>[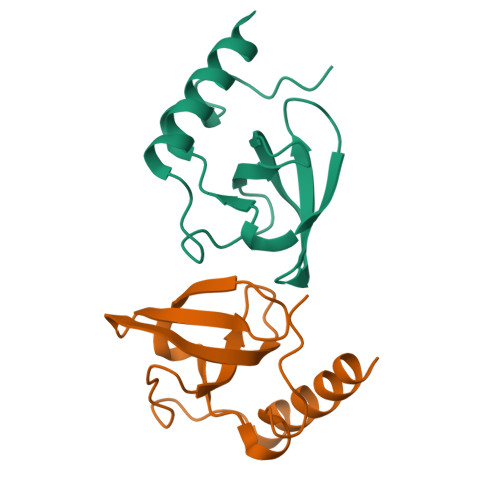2x]PVEEVMPVLEEKERSASYKPVFVTEITDDLHFYVQDVETGTQFQKLMENMRNDIASHPPVEGSYAPRRGEFCIAKFVDGEWYRARVEKVESPAKIHVFYIDYGNREVLPSTRLGTLSPAFSTRVLPAQATEYAFAFIQVPQDDDARTDAVDSVVRDIQNTQCLLNVEHLSAGCPHVTLQFADSKGDVGLGLVKEGLVMVEVRKEKQFQKVITEYLNAQESAKSARLNLWRYGDFRADDADEFGYSR> MILFKQATYFISLFATVSCGCLTQLYENAFFRGGDVASMYTPNAQYCQMRCTFHPRCLLFSFLPASSIND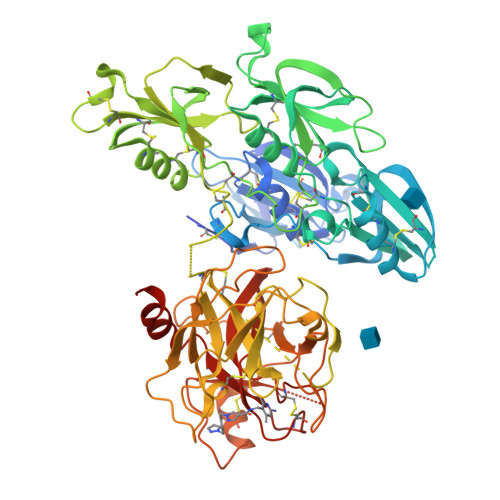MEKRFGCFLKDSVTGTLPKVHRTGAVSGHSLKQCGHQISACHRDIYKGVDMRGVNFNVSKVSSVEECQKRCTNNIRCQFFSYATQTFHKAEYRNNCLLKYSPGGTPTAIKVLSNVESGFSLKPCALSEIGCHMNIFQHLAFSDVDVARVLTPDAFVCRTICTYHPNCLFFTFYTNVWKIESQRNVCLLKTSESGTPSSSTPQENTISGYSLLTCKRTLPEPCHSKIYPGVDFGGEELNVTFVKGVNVCQETCTKMIRCQFFTYSLLPEDCKEEKCKCFLRLSMDGSPTRIAYGTQGSSGYSLRLCNTGDNSVCTTKTSTRIVGGTNSSWGEWPWQVSLQVKLTAQRHLCGGSLIGHQWVLTAAHCFDGLPLQDVWRIYSGILNLSDITKDTPFSQIKEIIIHQNYKVSEGNHDIALIKLQAPLNYTEFQKPICLPSKGDTSTIYTNCWVTGWGFSKEKGEIQNILQKVNIPLVTNEECQKRYQDYKITQRMVCAGYKEGGKDACKGDSGGPLVCKHNGMWRLVGITSWGEGCARREQPGVYTKVAEYMDWILEKTQSSDGKAQMQSPA> GSHMDSTTIQQNKDTLSQIVVFPTGNYDKNEANAMVNRLANIDGKYLNALKQNNLKIKLLSGKLTDEKE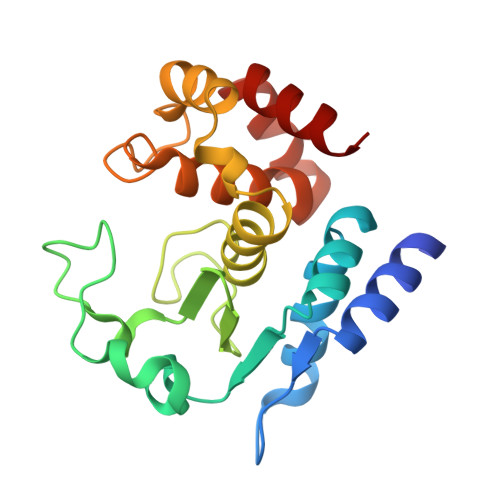YAYLKGVVPKGHEGTGKTWDDVPGLGGSTVALRIGFSNKGKGHDAINLELHATAHAIDHIVLNDISKSAQFKQIFAKEGRSLGNVNFLGVYPEEFFAESFAYYYLNQDTNSKLKSACPQTYSFLQNLAK3-[6-(but-3-en-1-yl)-7-oxo-6,7-dihydro-1H-pyrrolo[2,3-c]pyridin-4-yl]-N,N-dimethylbenzamide | C20 H21 N3 O2 | 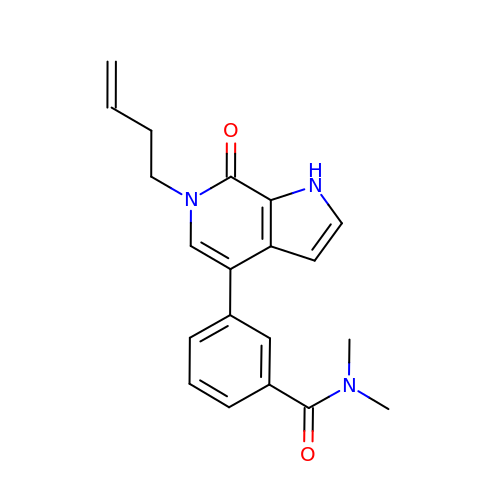VNCNIMOILJQAGJ-UHFFFAOYSA-N> TALTLVEQILAEFQLQEEDLKKVMRRMQKEMDRGLRLETHEEASVKMLPTYVRSTP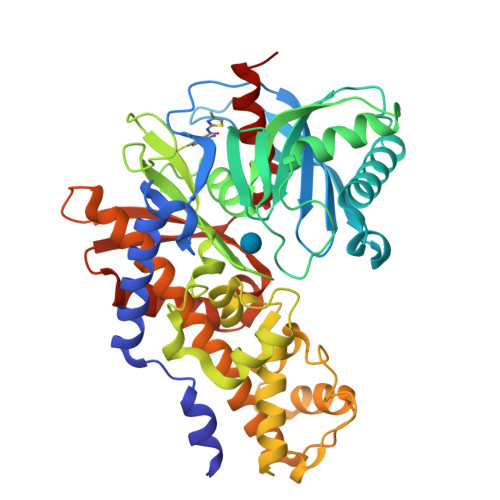EGSEVGDFLSLDLGGTNFRVMLVKVGEGEEGQWSVKTKHQMYSIPEDAMTGTAEMLFDYISECISDFLDKHQMKHKKLPLGFTFSFPVRHEDIDKGILLNWTKGFKASGAEGNNVVGLLRDAIKRRGDFEMDVVAMVNDTVATMISCYYEDHQCEVGMIVGTGCNACYMEEMQNVELVEGDEGRMCVNTEWGAFGDSGELDEFLLEYDRLVDESSANPGQQLYEKLIGGKYMGELVRLVLLRLVDENLLFHGEASEQLRTRGAFETRFVSQVESDTGDRKQIYNILSTLGLRPSTTDCDIVRRACESVSTRAAHMCSAGLAGVINRMRESRSEDVMRITVGVDGSVYKLHPSFKERFHASVRRLTPSCEITFIESEEGSGRGAALVSAVACKKACMLGQ> MDKSSIANKIEAYLGAKSDDSKIDQSLKADPSEVQYYGSGGDGYYLRKNICKITVNHSDSGTNDPCDRIPPPYGDNDQWKCAIILSKVSEKPENVFVPPRRQRMCINNLEKLNVDKIRDKHAFLADVLLTARNEGERIVQNHPDTNSSNVCNALERSFADIADIIRGTDLWKGTNSNLEQNLKQMFAKIRENDKVLQDKYPKDQNYRKLREDWWNANRQKVWEVITCGARSNDLLIKRGWRTSGKSNGDNKLELCRKCGHYEEKVPTKLDYVPQFLRWLTEWIEDFYREKQNLIDDMERHREECTSEDHKSKEGTSYCSTCKDKCKKYCECVKKWKSEWENQKNKYTELYQQNKNETSQKNTSRYDDYVKDFFKKLEANYSSLENYIKGDPYFAEYATKLSFILNSSDANNPSEKIQKNNDEVCNCNESGIASVEQEQISDPSSNKTCITHSSIKANKKKVCKHVKLGVRENDKDLRVCVIEHTSLSGVENCCCQDFLRILQENCSDNKSGSSSNGSCNNKNQEACEKNLEKVLASLTNCYKCDKCKSEQSKKNNKNWIWKKSSGKEGGLQKEYANTIGLPPRTQSLCLVVCLDEKGKKTQELKNIRTNSELLKEWIIAAFHEGKNLKPSHEKKNDDNGKKLCKALEYSFADYGDLIKGTSIWDNEYTKDLELNLQKIFGKLFRKYIKKNNTAEQDTSYSSLDELRESWWNTNKKYIWLAMKHGAGMNSTTCCGDGSVTGSGSSCDDIPTIDLIPQYLRFLQEWVEHFCKQRQEKVKPVIENCKSCKESGGTCNGECKTECKNKCEVYKKFIEDCKGGDGTAGSSWVKRWDQIYKRYSKYIEDAKRNRKAGTKNCGPSSTTNAAENKCVQSDIDSFFKHLIDIGLTTPSSYLSIVLDDNICGADKAPWTTYTTYTTTEKCNKETDKSKLQQCNTAVVVNVPSPLGNTPHGYKYACQCKIPTNEETCDDRKEYMNQWSCGSARTMKRGYKNDNYELCKYNGVDVKPTTVRSNSSKLDDKDVTFFNLFEQWNKEIQYQIEQYMTNTKISCNNEKNVLSRVSDEAAQPKFSDNERDRNSITHEDKNCKEKCKCYSLWIEKINDQWDKQKDNYNKFQRKQIYDANKGSQNKKVVSLSNFLFFSCWEEYIQKYFNGDWSKIKNIGSDTFEFLIKKCGNDSGDGETIFSEKLNNAEKKCKENESTNNKMKSSETSCDCSEPIYIRGCQPKIYDGKIFPGKGGEKQWICKDTIIHGDTNGACIPPRTQNLCVGELWDKRYGGRSNIKNDTKESLKQKIKNAIQKETELLYEYHDKGTAIISRNPMKGQKEKEEKNNDSNGLPKGFCHAVQRSFIDYKNMILGTSVNIYEYIGKLQEDIKKIIEKGTTKQNGKTVGSGAENVNAWWKGIEGEMWDAVRCAITKINKKQKKNGTFSIDECGIFPPTGNDEDQSVSWFKEWSEQFCIERLQYEKNIRDACTNNGQGDKIQGDCKRKCEEYKKYISEKKQEWDKQKTKYENKYVGKSASDLLKENYPECISANFDFIFNDNIEYKTYYPYGDYSSICSCEQVKYYEYNNAEKKNNKSLCHEKGNDRTWSKKYIKKLENGRTLEGVYVPPRRQQLCLYELFPIIIKNKNDITNAKKELLETLQIVAEREAYYLWKQYHAHNDTTYLAHKKACCAIRGSFYDLEDIIKGNDLVHDEYTKYIDSKLNEIFDSSNKNDIETKRARTDWWENEAIAVPNITGANKSDPKTIRQLVWDAMQSGVRKAIDEEKEKKKPNENFPPCMGVQHIGIAKPQFIRWLEEWTNEFCEKYTKYFEDMKSNCNLRKGADDCDDNSNIECKKACANYTNWLNPKRIEWNGMSNYYNKIYRKSNKESEDGKDYSMIMEPTVIDYLNKRCNGEINGNYICCSCKNIGENSTSGTVNKKLQKKETQCEDNKGPLDLMNKVLNKMDPKYSEHKMKCTEVYLEHVEEQLKEIDNAIKDY

VAR2CSA encoded by a subfamily of var genes from Plasmodium falciparum (P. falciparum) named as var2csa, plays a vital role in the cytoadherence of infected erythrocytes to the placenta. In this study, the VAR2CSA ectodomain from P. falciparum strain 3D7 (~306 kDa, containing six Duffy-binding-like (DBL) domains, N-terminal sequence (NTS), and multiple inter-domains (IDs))8 was recombinantly expressed and purified using the Sf9 insect cell secretory system. The cryo-EM structures of VAR2CSA ectodomain and its complex with CSA were determined at a resolution of 3.6 Å and 3.4 Å, respectively. In line with the previously proposed model, our structures showed that the core region is well-defined and covers NTS, DBL1X, DBL2X, ID2a, ID2b, DBL3X, ID3, and DBL4ε.

However, DBL5ε and DBL6ε formed a flexible wing region. As for the core region, DBL2X and DBL4ε stacked closely with ID2a, ID2b, and ID3, and formed the most stable core center, which served as a base for anchoring DBL3X and DBL1X at the top or bottom sites, respectively. First, the individual structures of four DBL domains (DBL1X, DBL2X, DBL3X, and DBL4ɛ) in the core region are quite similar to each other, with the typical “3 + 2” helix bundle shared. Uniquely, our structural study showed that CSA binding induced significant conformational changes to secure ligand binding, which was not reported by these two works.> MSLSWEIEELDREIGKIKKHSLILIHEEDASSRGKDILFYILSRKLKSDNLVGMFSISYPLQLIIRI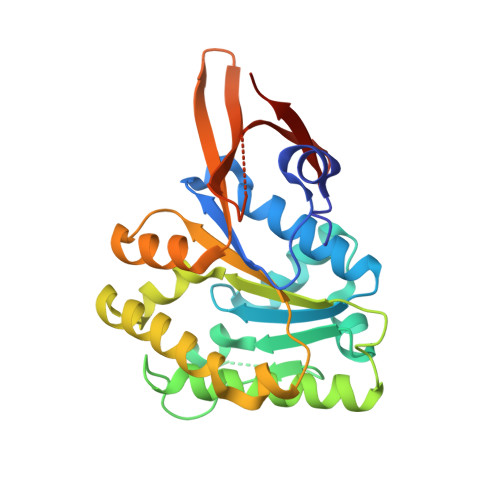LSRFGVDVIKYLENHRLAIVDTFGSFHGIKATMPGVWYLEGMLSSETLPIKYAKAVEDHKKVWMDLNLFEGRELYGFAISMSGYLEVFTPEETLRYLETSAEVRYGHPAYKKYPRGTNFWLWEGVKDKRVLLSVYRRADYVLKTRSSLGENGIKRELLVIKTPKPIEELVRFEYEFKGNEPKLRREGHHHHHH> GRVPDSIDYRKKGYVTPVKNQGQCGSCWAFSSAGALEGQLKKKTGKLLALSPQNLVDCVTENYG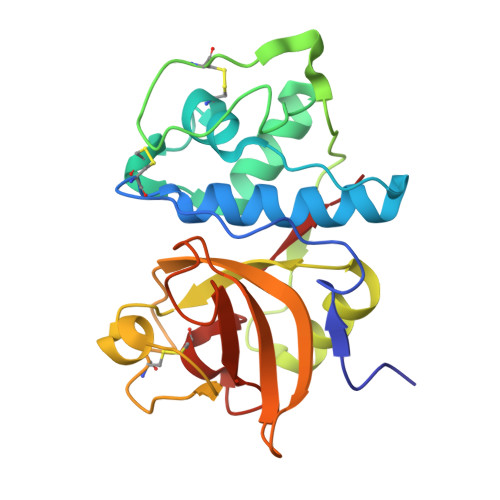CGGGYMTTAFQYVQQNGGIDSEDAYPYVGQDESCMYNATAKAAKCRGYREIPVGNEKALKRAVARVGPISVSIDASLASFQFYSRGVYYDENCDRDNVNHAVLVVGYGTQKGSKHWIIKNSWGESWGNKGYALLARNKNNACGITNMASFPKM Phosphorylated arginine residues (pArg) serve as a degradation signal that is recognized by the ClpC:ClpP (ClpCP) protease, a quasi-proteasomal particle critical for microbial protein quality control, stress tolerance, and pathogenicity (Trentini et al., 2016). ClpC carries out its quality control function by acting as an ATP-driven unfoldase that selects certain client proteins and translocates them into the protease compartment formed by ClpP. The ClpC protomer contains an amino-terminal domain (ClpCNTD), two AAA (ATPases associated with diverse cellular activities) domains termed D1 and D2, and a coiled coil (M domain) inserted into D1. In the active ClpC hexamer, the D1 and D2 domains form two stacked ATPase rings that power substrate unfolding and translocation.

Of note, the mycobacterial ClpC1 is targeted by a range of cyclic peptides that deregulate the ClpC1P1P2 complex. These antibiotics bind to the ClpC1NTD substrate receptor domain and thus have a pArg-like targeting function. The best characterized ClpC1NTD-directed antibiotic is CymA (Vasudevan et al., 2013), which binds to a hydrophobic pocket located in a remote position relative to the pArg-binding sites. The CymA binding pocket is highly conserved in ClpC1 unfoldases, but is absent in ClpC proteins from gram-positive bacteria, enabling selective targeting of the mycobacterial protease. Guided by structural data (Vasudevan et al., 2013), we prepared a series of CymA-like cyclic peptides and identified sCym-1 as a high affinity ClpC1NTD ligand (KD = 0.81 μM). A co-crystal structure obtained at 1.7 Å resolution confirmed that the sCym-1 mimetic adopts the same binding mode as the native CymA antibiotic. Moreover, the crystal structure revealed a possible linker attachment site to synthesize BacPROTAC-2, in which sCym-1 is linked to biotin. The respective alanine side chain does not contribute to the sCym-1:ClpC1NTD interface. When tested in our biochemical assay, the sCym-1-based degrader stimulated removal of the mSA model substrate to similar extents as its pArg counterpart, indicating that derivatives of the CymA antibiotic can be repurposed as BacPROTAC components. Importantly, these data also show that various ClpC1NTD binders can be exploited to develop chemical adaptors for targeted protein degradation.

> MFERFTDRARRVVVLAQEEARMLNHNYIGTEHILLGLIHEGEGVAAKSLESLGISLEGVRSQVEEIIGQGQQAPSGHIPFTPRAKKVLELSLREALQLGHNYIGTEHILLGLIREGEGVAAQVLVKLGAELTRVRQQVIQLLSGYQGKLEHHHHHH;> WXAFVLI>[4x]MDTWKVGPVELKSRLILGSGKYEDFGVMREAIAAAKAEVVTVSVRRVELKAPGHVGLLEALEGVRLLPNTAGARTAEEAVRLARLGRLLTGERWVKLEVIPDPTYLL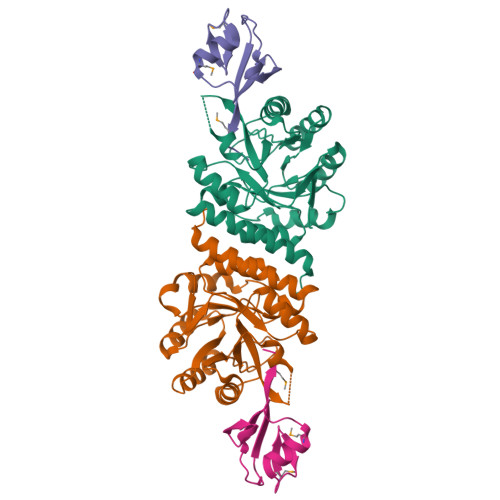PDPLETLKAAERLIEEDFLVLPYMGPDLVLAKRLAALGTATVMPLAAPIGSGWGVRTRALLELFAREKASLPPVVVDAGLGLPSHAAEVMELGLDAVLVNTAIAEAQDPPAMAEAFRLAVEAGRKAYLAGPMRPREAASPSSPVEGVPFTPTGPRPGRGPQ;>MVWLNGEPRPLEGKTLKEVLEEMGVELKGVAVLLNEEAFLGLEVPDRPLRDGDVVEVVALMQGG[4x]>ALFTGIIPPVSTIFTADGQLDKPGTAALIDDLIKAGVDGLFFLGSGGEFSQLGAEERKAIARFAIDHVDRRVPVLIGTGGTNARETIELSQHAQQAGADGIVVINPYYWKVSEANLIRYFEQVADSVTLPVMLYNFPALTGQDLTPALVKTLADSRSNIIGIKDTIDSVAHLRSMIHTVKGAHPHFTVLCGYDDHLFNTLLLGGDGAISASGNFAPQVSVNLLKAWRDGDVAKAAGYHQTLLQIPQMYQLDTPFVNVIKEAIVLCGRPVSTHV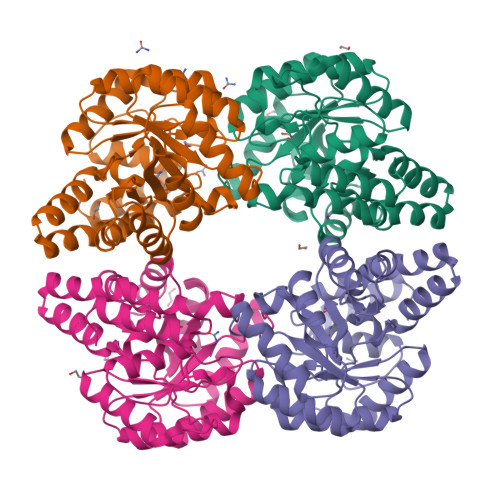LPPASPLDEPRKAQLKTLLQQLKLC[4x]> GEDKHDIVDG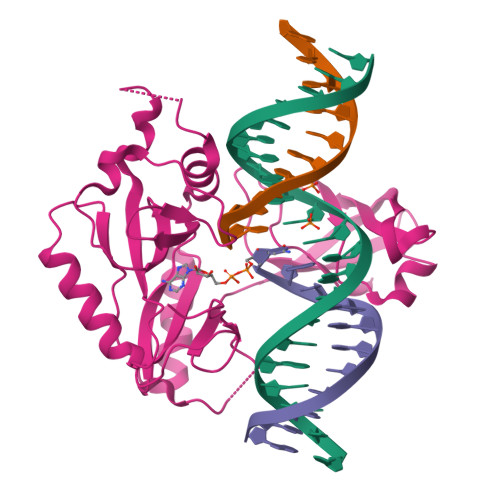LQLAKQYGHSRQDINIAEYWVSEKLDGIRARWDGTELRTRNNNKIDAPAWFTANWPKATIDGELWIARGQFERTASIVLSKLTSVAPQSVAGSLPRTESTVDAMTATHSLPSKRWAKVRFMAFDMPVAGQSFDSRLNMLNNLKEATPNPTFAVVSQFTLSSVNALEEKLEQVTLSGGEGLMLHHKKAFYHSGRSDKLIKVKQFEDAEAKVLAHFAGKGKFKGMMGSLLVETPAGVQFKLGTGFSEKERRAPPAVGSWVTFKFYGVTKNGKPRFASFLRVRPPSDLPK> MGSSHHHHHHSSGENLYFQGRPMSSMNPEYDY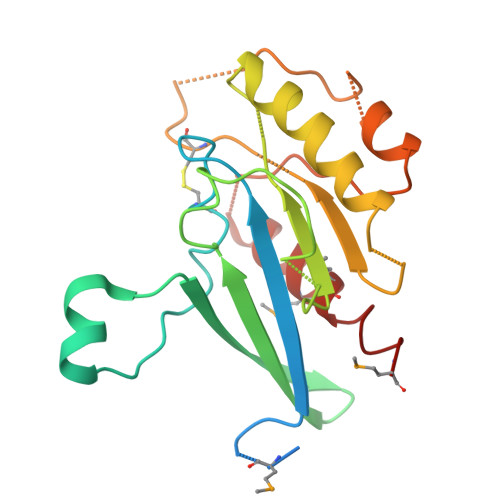LFKLLLIGDSGVGKSCLLLRFADDTYTESYISTIGVDFKIRTIELDGKTIKLQIWDTAGQERFRTITSSYYRGAHGIIVVYDVTDQESFNNVKQWLQEIDRYASENVNKLLVGNKCDLTTKKVVDYTTAKEFADSLGIPFLETSAKNATNVEQSFMTMAAEIKKRMG N-[(2R)-2-{[(7-chloro-2-oxo-1,2-dihydroquinolin-6-yl)sulfonyl]amino}-2-(2-methoxyphenyl)acetyl]-N-[(thiophen-2-yl)methyl]glycine | C25 H22 Cl 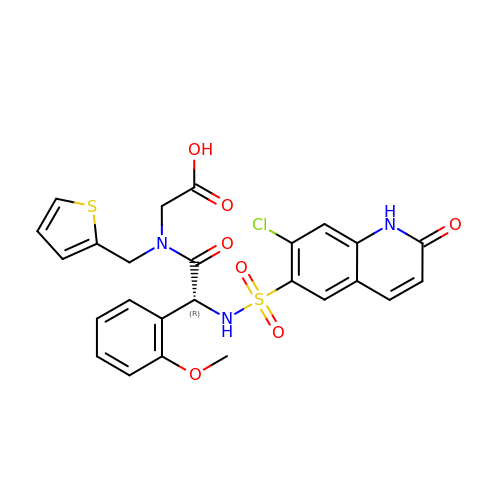N3 O7 S2 | AZINZNCYZJSBMU-XMMPIXPASA-N>[6x]MTVTDIILIHGALNRGACYDAVVPLLEARGYRVHAPDLTGHTPGDGGHLSVVDMEHYTRPVADILARAEGQSILLGHSLGGASISWLAQHHPDKVAGLIYLTA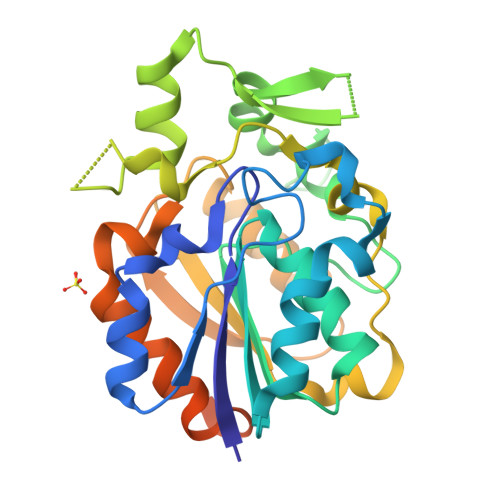VLTAPGVTPETFVLPGEPNRGTPHALDLIQPVDEGRGLQADFSRLERLREVFMGDYPGEGMPPAEHFIQTQSTVPFGTPNPMEGRALEIPRLYIEALDDVVLPIAVQRQMQKEFPGPVAVVSLPASAAPYYSMPERLAEAIADFADAPAEYRQTATKAGPDRPAGADGGRADRADLPLEHHHHHH>MAMANNSSVANKVCLIVIDGWGVSEDPYGNAILNAQTPVMDKLCSGNWAQIEAHGLHVGLPEGLMGNSEVGHLNIGAGRVIYQDIVRINLAVKNNKFVTNESLVDACDRAKNGNGRLHLAGLVSDGGVHSHIDHMFALVKAIKELGVPELYLHFYGDGRDTSPNSGVGFLEQTLEFLEKTTGYGKLATVVGRYYAMDRDNRWERINVAYEAMIGGVGETSDEAGVVEVVRKRYAADETDEFLKPIILQGEKGRVQNDDTIIFFDYRADRMREISAAMGMDRYKDCNSKLAHPSNLQVYGMTQYKAEFPFKSLFPPASNKNVLAEWLAEQKVSQFHCAETEKYAHVTFFFNGGLEKQFEGEERCLVPSPKVATYDLQPEMSAAGVADKMIEQLEAGTHPFIMCNFAPPDMVGHTGVYEAAVKACEATDIAIGRIYEATQKHGYSLMVTADHGNAEKMKAPDGGKHTAHTCYRVPLTLSHPGFKFVDPADRHPALCDVAPTVLAIMGLPQPAEMTGVSIVQKIKLAAALEHHHHHHHHHH[2x];>XYDYPGDHCYLYGTX[2x]

In all vertebrates, cofactor-dependent phosphoglycerate mutase (dPGM) is a 2, 3-bisphophoglycerate cofactor–utilizing homodimer consisting of 23-kDa subunits, while the parasitic enzyme is a 56-kDa monomer cofactor-independent enzyme consisting of a phosphatase domain connected by a flexible hinge to the phosphotransferase domain. In dPGM, an active site phosphohistidine (H10) equilibrates the phosphate between the 2 and 3 positions of glyceric acid, while in cofactor-independent phosphoglycerate mutase (iPGM), a transition metal ion–activated serine (S86) mediates the phosphate transfer. We previously discovered ipglycermide, a potent inhibitor of iPGM, from a large combinatorial cyclic peptide library. Our results show that the high-affinity binding of ipglycermide to iPGMs freezes these structurally dynamic enzymes into an inactive, stable complex.

To gain structural insight into the molecular interactions of the C-terminus of ipglycermides with iPGM, we established co-crystal structures using analogs, Ce-2 Tyr7Phe and Ce-1 Cys14NHOH (Ce-1 NHOH), respectively, retaining Cys14 or replacing it with NHOH, an oxidation-insensitive and solid-phase peptide synthesis (SPPS)-accessible metal-ion–coordinating ligand. Using our established crystallization conditions, supplemented with 2-mM tris(2-carboxyethyl)phosphine for Ce-2 Tyr7Phe–containing complexes, we were able to obtain crystals diffracting to 2.1 Å and 1.80 Å for Ce-2 Tyr7Phe and Ce-1 NHOH, respectively, bound to C. elegans iPGM. The electron density maps for these complexes were clearly defined, and all atoms for the ipglycermides could be modeled except for the Ce-1 NHOH solvent-exposed Tyr11 side chain. The “core” region of the peptide (Tyr1-Tyr11) forms hydrogen-bond interactions with N85, Q101, D102, and R289 like Ce-2d. However, residues 12 to 14 of Ce-2 Tyr7Phe and Ce-1 NHOH display nonoverlapping conformations resulting from differences in Zn2+ coordination. The C-terminal Thr13-hydroxamate residue side chain forms an interaction with E87, which appears to constrain this portion of the peptide and permits a bidentate interaction from the carbonyl (2.15 Å) and hydroxyl (2.30 Å) to a Zn2+. In addition, the Thr13 hydroxyl forms a hydrogen bond with the active site S86 that is coordinated to the second Zn2+. Notably, the sulfur atom of Cys14 is positioned in a nearly identical region as the Thr13/hydroxamate carbonyl in the iPGM⋅Ce-1 NHOH structure. Despite these conformational displacements, the Thr13 side-chain hydroxyl adopts a similar spatial position in both structures, thereby maintaining the hydrogen-bond interaction with the phosphatase domain E87 γ-carboxylate. Whereas the Ce-1 NHOH analog displays similar pan-ortholog inhibitory potency as Ce-1 and Ce-2, thus the Thr13-hydroxamic acid moiety acts as rather selective bio-isostere for the Cys14 thiolate of ipglycermide.>GKLSLQDVAELIRARACQRVVVMVGAGISTPSGIPDFRSPGSGLYSNLQQYDLP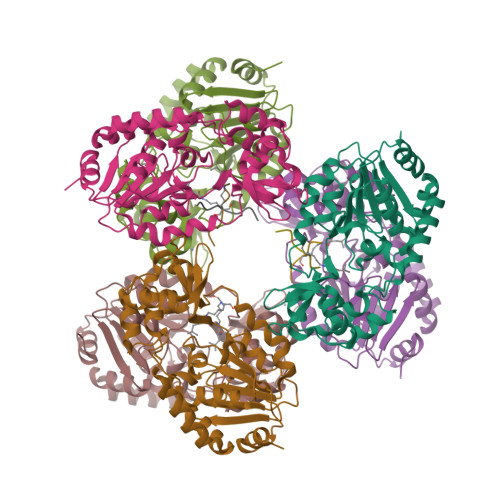YPEAIFELPFFFHNPKPFFTLAKELYPGNYKPNVTHYFLRLLHDKGLLLRLYTQNIDGLERVSGIPASKLVEAHGTFASATCTVCQRPFPGEDIRADVMADRVPRCPVCTGVVKPDIVFFGEPLPQRFLLHVVDFPMADLLLILGTSLEVEPFASLTEAVRSSVPRLLINRDLVGPLAWHPRSRDVAQLGDVVHGVESLVELLGWTEEMRDLVQRETGKL[6x];>[4x]TRSGKVMR> MGHHHHHHAAKNAVKKNKRVLRGSVKEANYFVEGEASAATIDAVLNDVDLVITKIDADEIAALAGKLNGLTVADEIKN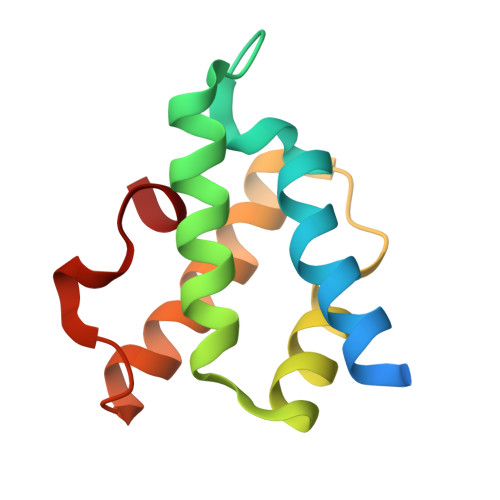VWKEEVSRLVGAGKLKEGDIKALVA Tom70 is one of the major import receptors in the translocase of the outer membrane (TOM) complex that recognizes and mediates the translocation of mitochondrial preproteins from the cytosol into the mitochondria in a chaperone-dependent manner. It contains an N-terminal transmembrane domain and tetratricopeptide repeat (TPR) motifs in its cytosolic segment. The C-terminal TPR motifs recognize the internal mitochondrial targeting signals (MTSs) of preproteins, and the N-terminal TPR clamp domain serves as a docking site for multichaperone complexes that contain preprotein. In line with this, the mitochondrial outer membrane protein Tom70 (encoded by TOMM70) is a high-confidence interactor of ORF9b in both SARS-CoV-1 and SARS-CoV-2 interaction maps, and it acts as a host-dependency factor for SARS-CoV-2.

Further, upon coexpression in bacterial cells, we were able to copurify the ORF9b-Tom70 protein complex, which indicates a stable complex. Using cryo-EM, we obtained a 3-Å structure of a region of ORF9b binding to the active site of Tom70. Obtained cryo-EM density allowed us to build atomic models for residues 109 to 600 of human Tom70 and residues 39 to 76 of SARS-CoV-2 ORF9b. ORF9b makes extensive hydrophobic interactions at the pocket on Tom70 that have been implicated in its binding to MTS, with the total buried surface area at the interface being quite extensive—~2000 Å2. In addition to the mostly hydrophobic interface, four salt bridges further stabilize the interaction. On interaction with ORF9b, the interacting helices on Tom70 move inward to tightly wrap around ORF9b as compared with previously crystallized yeast Tom70 homologs. Notably, we found that ORF9b is in a markedly different conformation than previously visualized. Furthermore, we had previously identified two infection-driven phosphorylation sites on ORF9b, S50 and S53 (17), which map to the region on ORF9b buried deep in the Tom70 binding pocket (yellow). S53 contributes two hydrogen bonds to the interaction with Tom70 in this overall hydrophobic region.

> NSLDRAQAAKNKGNKYFKAGKYEQAIQCYTEAISLCPTEKNVDLSTFYQNRAAAFEQLQKWKEVAQDCTKAVELNPKYVKALFRRAKAHEKLDNKKECLEDVTAVCILEGFQNQQSMLLADKVLKLLGKEKAKEKYKNREPLMPSPQFIKSYFSSFTDDIISQPMLKGEKSDEDKDKEGEALEVKENSGYLKAKQYMEEENYDKIISECSKEIDAEGKYMAEALLLRATFYLLIGNANAAKPDLDKVISLKEANVKLRANALIKRGSMYMQQQQPLLSTQDFNMAADIDPQNADVYHHRGQLKILLDQVEEAVADFDECIRLRPESALAQAQKCFALYRQAYTGNNSSQIQAAMKGFEEVIKKFPRCAEGYALYAQALTDQQQFGKADEMYDKCIDLEPDNATTYVHKGLLQLQWKQDLDRGLELISKAIEIDNKCDFAYETMGTIEVQRGNMEKAIDMFNKAINLAKSEMEMAHLYSLCDAAHAQTEVAKKYGLKPPTL;> MDPKISEMHPALRLVDPQIQLAVTRMENAVGRDQNNVGPKVYPIILRLGSPLSLNMARKTLNSLEDKAFQLTPIAVQMTKLATTEELPDEFVVVTVK> HMPAFLSKLWTLVEETHTNEFITWSQNGQSFLVLDEQRFAKEIL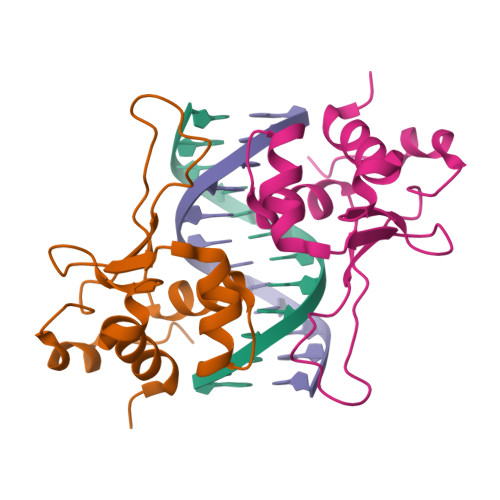PKYFKHNNMASFVRQLNMYGFRKVVHIDSGIVKQERDGPVEFQHPYFKQGQDDLLENIKRKVSSSK>DDSFPIAGIYDTTTDNKCSIKTAVAKNMLDPITGQKLLEAQAATGGIVDLLSRERYSVHKAMERGLIENTSTQRLLNAQKAFTGIEDPVTKKRLSVGEAVQKGWMPRESVLPHLQVQHLTGGLIDPKRTGRIPIQQALLSGMISEELAQLLQDESSYEKDLTDPISKERLSYKEAMGRCRKDPLSGLLLLPAA[2x]

The plakin protein envoplakin is upregulated during keratinocyte terminal differentiation, and interacts with the closely related protein periplakin to initiate cornified envelope formation. Although their architectures have diverged, all plakin proteins except periplakin contain at least one plakin repeat domain (PRD), which constitutes a conserved node that links cell junctions directly to cytoskeletal frameworks, disruption of which has dire physiological consequences. Of all the plakin proteins, envoplakin is the only member to contain a single PRD module, which is connected to a central coiled coil region through a linker domain. The structure reveals a basic groove that can accommodate acidic patches on the cylindrical surface of monomeric or multimeric intermediate filament proteins.

The construct boundaries were selected based on sequence alignment, and the resulting structure was solved to 1.6 Å resolution by single-wavelength anomalous dispersion. The asymmetric unit was comprised of two PRD molecules designated ‘a' and ‘b'. Models comprising residues Asp1822 to Ala2014 were built and refined to R and Rfree factors of 16.8% and 20.5%, respectively. The two envoplakin PRD molecules in the asymmetric unit are similar, superimposing with a root mean square (r.m.s.) deviation of 1.1 Å for 183 aligned Cα atoms. The envoplakin PRD structure has two lobes and contains 4.5 copies of the canonical 38 amino-acid plakin repeat (PR) motif followed by a C-terminal hairpin turn. A novel conformation is found in envoplakin's PR4 motif, where a long loop is found instead of the canonical β-hairpin. A striking feature observed in envoplakin is the non-canonical helical structure and distinctive kink of H2 in PR2. The electrostatic potential of the envoplakin PRD surface reveals a polarized protein with a highly positively charged groove. One basic flank is formed by H2 of PR1 and H2 of PR2, another by S1, S2 and H2 of PR3, while the elongated loop of PR4 forms a cap. This surface area contains a deep groove which is ∼23 Å long and 10 Å wide. The groove is delineated by Arg1952 and Lys1994 at one end, and Lys1901 and Arg1914 at the other extremity, while Arg1876 and Arg1895 lie centrally.> SMDAFEKVRTKLETQPQEEYEIINVEVKHGGFVYYQEGCCLVRSKDEEADNDNYEVLFNLEELKLDQPFIDCIRVAPDEKYVAAKIRTEDSEASTCVIIKLSDQPVMEASFPNVSSFEWVKDEEDEDVLFYTFQRNLRCHDVYRATFGDNKRNECFYTEKDPSYFVFLYLTKDSRFLTINIMNKTTSEVWLIDGLSPWDPPVLIQKRIHGVLYYVEHRDDELYILTNVGEPTEFKLMRTAADTPAIMNWDLFFTMKRNTKVIDLDMFKDHCVLFLKHSNLLYVNVIGLADDSVRSLKLPPWACGFIMDTNSDPKNCPFQLCSPIRPPKYYTYKFAEGKLFEETGHEDPITKTSRVLRLEAKSKDGKLVPMTVFHKTDSEDLQKKPLLVHVYGAYGMDLKMNFRPERRVLVDDGWILAYCHVRGGGELGLQWHADGRLTKKLNGLADLEACIKTLH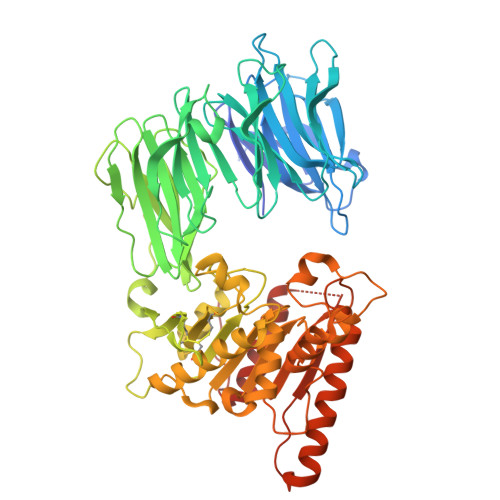GQGFSQPSLTTLTAFSAGGVLAGALCNSNPELVRAVTLEAPFLDVLNTMMDTTLPLTLEELEEWGNPSSDEKHKNYIKRYCPYQNIKPQHYPSIHITAYENDERVPLKGIVSYTEKLKEAIAEHAKDTGEGYQTPNIILDIQPGGNHVIEDSHKKITAQIKFLYEELGLDSTSVFEDLKKYLKF> MPAPAATYERVVYKNPSEYHYMKVCLEFQDCGVGLNAAQFKQLLISAVKDLFGEVDAALPLDILTYEEKTLSAILRICSSGL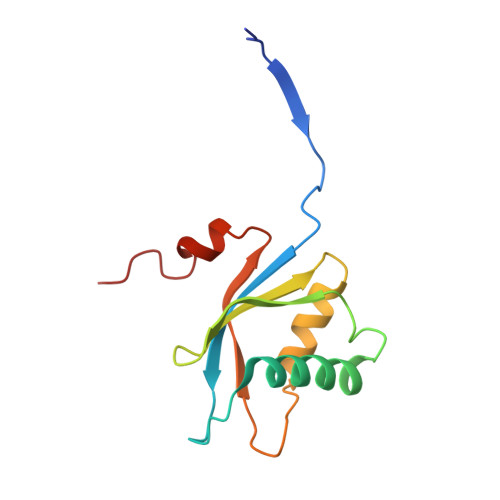VKLWSSLTLLGSYKGKKCAFRVIQVSPFLLALSGNSRELVLD> MGMWKWLVIASLVWPALSLRNVYDMKIECPHTVSFGENSVIGYVELPPMPLADTAQMVPESSCSMDNHQSINTITKYTQVIWRGKADPGQSSQNSFETVSTEVDLKGTCVLKHKMVEESYRSRKSITCYDLSCNSTFCKPTLYMIVPIHACNMMKSCLIALGPYRVQVVYERTYCMTGVLIEGKCFVPDQSVVSIIKHGIFDIASVHVVCFFVAVKGNTYKLFEQVKKSFESTCNDTENKVQGYYICIVGGNSAPIYVPTLDDFRSMEAFTGIFKSPHGEDHDLAGEEIASYSIVGPANAKVPHSASSDTLSLIAYSGIPSYSSLSILTSSTDAKHVFSPGLFPKLNHTNCDKSAIPLTWTGMIDLPGYYE

The outer membrane of the hantavirus envelope displays a lattice of two glycoproteins, Gn and Gc, which orchestrate host cell recognition and entry. The hantaviral envelope comprises a lipid bilayer with an outer proteinaceous shell of two glycoproteins, Gn and Gc, which are synthesized as a single polyprotein precursor (GPC). Fitting of the PUUV Gn ectodomain crystal structure into a low-resolution reconstruction of the mature hantaviral glycoprotein spike complex revealed that the Gn is membrane distal and likely shields hydrophobic fusion loops on the Gc. Following receptor recognition, hantaviruses undergo clathrin-mediated endocytosis, and the viral genome is delivered into the cytoplasm following Gc-mediated fusion of viral and host membranes, a process triggered by the acidic pH of late endosomes or lysosomes.

Here, we sought to understand the architecture of the HTNV glycoprotein envelope and report the crystal structure of the Gn ectodomain to 2.15-Å resolution. A construct comprising HTNV Gn ectodomain residues 18 to 371 was crystallized under a condition comprising equal volumes of the protein in sample buffer (10 mM Tris, pH 8.0, 150 mM NaCl) and precipitant (1.6 M ammonium sulfate, 0.1 M citrate pH 4.0). The one molecule of HTNV Gn observed in the asymmetric unit displays a β-sandwich fold stabilized by seven disulfide bonds and composed of five antiparallel β-sheets and six α-helices. While PUUV Gn and HTNV Gn share limited amino acid sequence identity (44%) and similarity (64%) over the crystallized region, HTNV Gn exhibits a high level of structural homology to PUUV Gn (1.3-Å root-mean-square deviation [RMSD] over 315 Cα atoms), corroborating the hypothesis that the Gn fold is a well-conserved feature among hantaviruses. We note that two loops (residues 190 to 197 and residues 281 to 289) were not ordered well enough for model building in the HTNV Gn structure. HTNV Gn was crystallized at acidic pH, and analysis of crystallographic packing revealed a compact tetrameric assembly, termed herein the acidic Gn tetramer. Residues 82 to 96 appear to play a chief role in the construction of this higher-order assembly, forming a β-hairpin that interlocks into a pocket formed on the neighboring Gn protomer. Each of the four equivalent protomeric interfaces of the acidic Gn tetramer is extensive, occluding approximately 1,850 Å2 of solvent-accessible surface, and reinforced by 16 hydrogen bonds. Indeed, although the acidic tetramer more closely resembles fit 2 than fit 1, it is far more compact than either fit and exhibits a width reduced by approximately one-third (50 Å). We present a model predicting how the Gn both shields the hydrophobic fusion loops on the Gc at neutral pH and dissociates from the Gc during Gc-mediated fusion in endosomal compartments.>LNCGQVDSKMKPCLTYVQGGPGPSGECC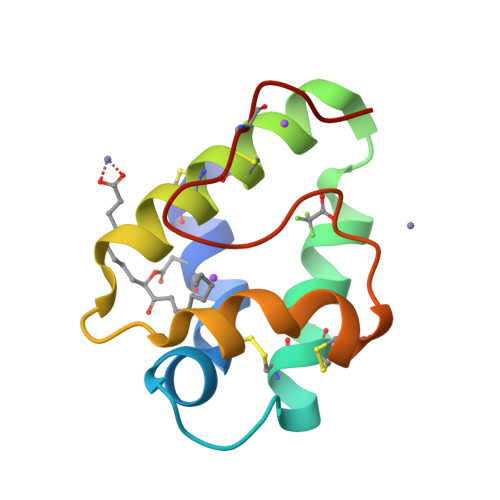NGVRDLHNQAQSSGDRQTVCNCLKGIARGIHNLNLNNAASIPSKCNVNVPYTISPDIDCSRIY[2x]> MFKAQATFSRYSAAVSLLLLFSGAAQAAPQSITTLPLQPDGENRWRLPAGEYQGQFTIEQPMQLRCEPGAVIQSQGQGSSLLISAPDVLVEGCTLYEWGSDLTAMDSAVFILPAAERAQISNNRMRGPGFGVFVDGTRDVQVIGNEIDGDAGVRSQDRGNGIHLFAVSGARVLHNHVRNARDGIYIDTSNGNHLEGNVIEDVRYGVHYMFANENSLIDNVTRRTRTGYALMQSRKLTVTGNRSEQDQNYGILMNYITYSTITGNFVSDVQRGDTGGDSMISGGEGKALFIYNSLFNTIENNHFEKSSLGIHLTAGSEDNRISGNAFVGNQQQVKYVASRTQEWSVDGRGNYWSDYLGWDRNNDGLGDIAYEPNDNVDRLLWLYPQVRLLMNSPSIEVLRWVQRAFPVIKSPGVQDSHPLMKLPTEKLLTEKQEPTS;>MNAVEIQGVSQRYGSMTVLHDLNLNLGEGEVLGLFGHNGAGKTTSMKLILGLLSPSEGQVKVLGRAPNDPQVRRQLGYLPENVTFYPQLSGRETLRHFARLKGAALTQVDELLEQVGLAHAADRRVKTYSK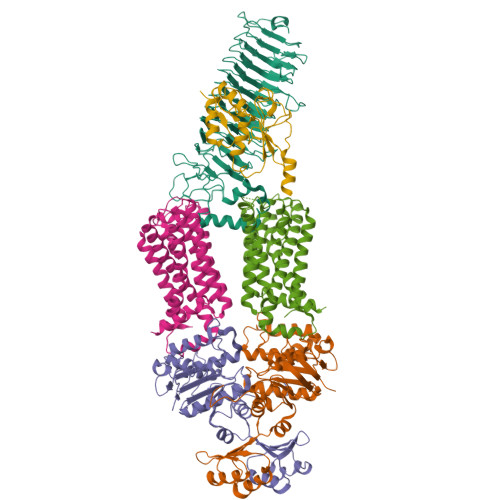GMRQRLGLAQALLGEPRLLLLDEPTVGLDPIATQDLYLLIDRLRQRGTSIILCSHVLPGVEAHINRAAILAKGCLQAVGSLSQLRAEAGLPVRIRASGISERDSWLQRWTDAGHSARGLSESSIEVVAVNGHKLVLLRQLLGEGEPEDIEIHQPSLEDLYRYYMERAGDVRAQEGRL[2x];>[2x]MNQVWNIARKELSDGLRNRWLLAISLLFAVLAVGIAWLGAAASGQLGFTSIPATIASLASLATFLMPLIALLLAYDAIVGEDEGGTLMLLLTYPLGRGQILLGKFVGHGLILALAVLIGFGCAALAIALLVEGVELGMLFWAFGRFMISSTLLGWVFLAFAYVLSGKVNEKSSAAGLALGVWFLFVLVFDLVLLALLVLSEGKFNPELLPWLLLLNPTDIYRLINLSGFEGSGSAMGVLSLGADLPVPAAVLWLCLLAWIGVSLLLAYAIFRRRLT;> MNALHRIGAGTLLAVLLAFGLTGCGEKEEVQQSLEPVAFHDSDECHVCGMIITDFPGPKGQAVEKRGVKKFCSTAEMLGWWLQPENRLLDAKLYVHDMGRSVWEKPDDGHLIDATSAYYVVGTSLKGAMGASLASFAEEQDAKALAGMHGGRVLRFEEIDQALLQEAASMQHGGMHDHAPNGAHNAHAGH>MSTAITRQIVLDTETTGMNQIGAHYEGHKIIEIGAVEVVNRRLTGNNFHVYLKPDRLVDPEAFGVHGIADEFLLDKPTFAEVADEFMDYIRGAELVIHNAAFDIGFMDYEFSLLKRDIPKTNTFCKVTDSLAVARKMFPGKRNSLDALCARYEIDNSKRTLHGALLDAQILAEVYLAMTGGQTSMA[2x];>[2x]MYDWNIAAKSQEERDKVNVDLAASGVAYKERLNIPVIAEQVAREQPENLRTYFMERLRHYRQLSLQLPKGS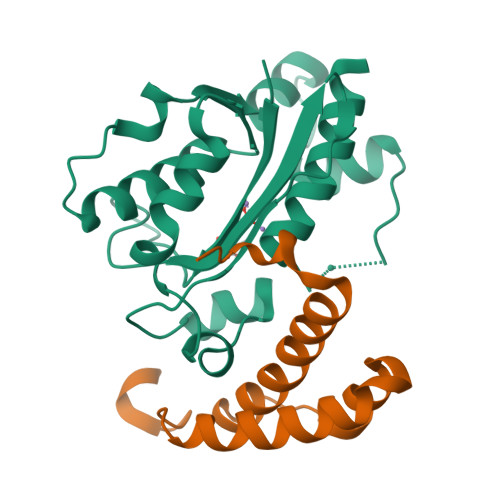DPAYQKDDAVKK>MVSGGTFNAGVEKIRPGIYTNFKAAAAERTKAGERGTVALPLAASWGAAKEFVEINKEEDVEKKLGLSLAHQSFLLLRETLKLAKTVLVYRLNDGIKATATLATDVVVTAKYGGIVGNSITIKVDENVVDSSKKDVTTYLNEVAVDKQVVGTASELIDSNYVSFKTTSTSELQQSSGTTLVGGTDQPVTNLDYTQFLVSAEGEYFDTIAFPVSSSDVALKTSFVSFVKRMRDEQGVKIKGVVANMPADYEGIINVRNGVTLRDGTILEPHQVVAWVAGADASASMLKSNTFVKYDGAIDATPRLANDEAEEALQNGEFVLTFDARDKAVYVEQDLNSLTTFSKEKSSKFRKNKISRILDGINNDTRRNILDAIKERKDANTDIPADENGVQFILSMQTAYLNELQDSGAITNFDSTADITVSLNNNVDGFIVNQSIEPVDSGEKFYFTTEVKLEHHH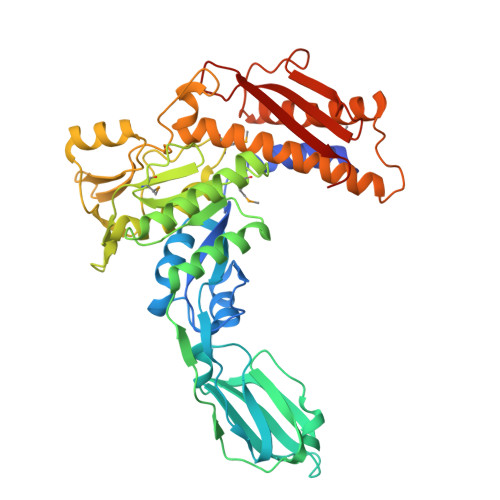HHH[6x]>MTNLSDQTQQIVPFIRSLLMPTTGPASIPDDTLEKHTLRSETSTYNLTVGDTGSGLIVFFPGFPGSIVGAHYTLQGNGNYKFDQMLLTAQNLPASYNYCRLVSRSLTVRSSTLPGGVYALNGTINAVTFQGSLSELTDVSYNGLMSATANINDKIGNVLVGEGVTVLSLPTSYDLGYVRLGDPIPAIGLDPKMVATCDSSDRPRVYTITAADDYQFSSQYQPGGVTITLFSANIDAITSLSVGGELVFRTSVHGLVLGATIYLIGFDGTTVITRAVAANNGLTTGTDNLMPFNLVIPTNEITQPITSIKLEIVTSKSGGQAGDQMSWSARGSLAVTIHGGNYPGALRPVTLVAYERVATGSVVTVAGVSNFELIPNPELAKNLVTEYGRFDPGAM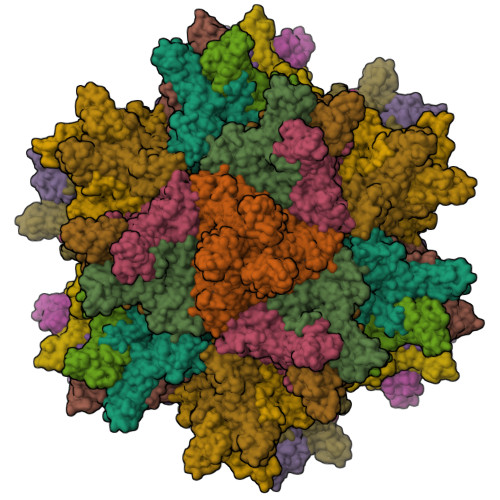NYTKLILSERDRLGIKTVWPTREYTDFREYFMEVADLNSPLKIAGAFGFKDIIRAIRRIAV[20x]>HGHSSSDPVYPCGICTNEVNDDQDAILCEASCQKWFHRICTGMTETAYGLLTAEASAVWGCDTCMAD[2x];>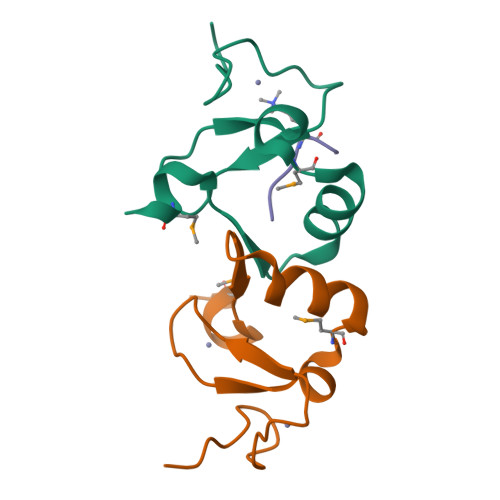 ARTKQTAR> SQMDISNFYIRDYMDFAQNKGIFQAGATNIEIVKKDGSTLKLPEVPFPDFSPVANKGSTTSIGGAYSITATHNTKNHHSVATQNWGNSTYKQTDWNTSHPDFAVSRLDKFVVETRGATEGADISLSKQQALERYGVNYKGEKKLIAFRAGSGVVSVKKNGRITPFNEVSYKPEMLNGSFVHIDDWSGWLILTNNQFDEFNNIASQGDAGSALFVYDNQKKKWVVAGTVWGIYNYANGKNHAAYSKWNQTTIDNLKNKYSYNVDMSGAQVATIENGKLTGTGSDTTDIKNKDLIFTGGGDILLKSSFDNGAGGLVFNDKKTYRVNGDDFTFKGAGVDTRNGSTVEWNIRYDNKDNLHKIGDGTLDVRKTQNTNLKTGEGLVILGAEKTFNNIYITSGDGTVRLNAENALSGGEYNGIFFAKNGGTLDLNGYNQSFNKIAATDSGAVITNTSTKKSILSLNNTADYIYHGNINGNLDVLQHHETKKENRRLILDGGVDTTNDISLRNTQLSMQGHATEHAIYRDGAFSCSLPAPMRFLCGSDYVAGMQNTEADAVKQNGNAYKTNNAVSDLSQPDWETGTFRFGTLHLENSDFSVGRNANVIGDIQASKSNITIGDTTAYIDLH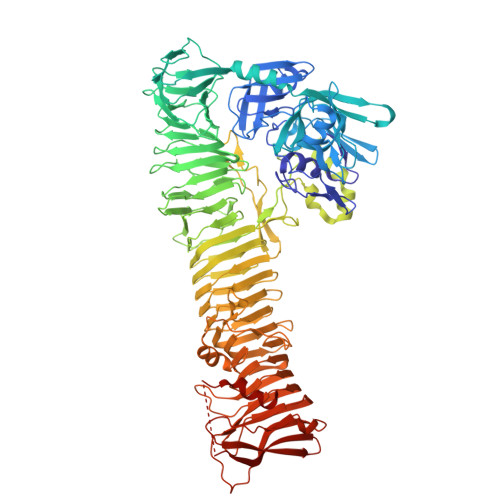AGKNITGDGFGFRQNIVRGNSQGETLFTGGITAEDSTIVIKDKAKALFSNYVYLLNTKATIENGADVTTQSGMFSTSDISISGNLSMTGNPDKDNKFEPSIYLNDASYLLTDDSARLVAKNKASVVGDIHSTKSASIMFGHDESDLSQLSDRTSKGLALGLLGGFDVSYRGSVNAPSASATMNNTWWQLTGDSALKTLKSTNSMVYFTDSANNKKFHTLTVDELATSNSAYAMRTNLSESDKLEVKKHLSGENNILLVDFLQKPTPEKQLNIELVSAPKDTNENVFKASKQTIGFSDVTPVITTRETDDKITWSLTGYNTVANKEATRNAAALFSVDYKAFLNEVN> PPRPSSGELWGIHLMPPRILVECLLPNGMIVTLECLREATLITIKHELFKEARKYPLHQLLQDESSYIFVSVTQEAEREEFFDETRRLCDLRLFQPFLKVIEPVGNREEKILNREIGFAIGMPVCEFDMVKDPEVQDFRRNILNVCKEAVDLRDLNSPHSRAMYVYPPNVESSPELPKHIYNKLDKGQIIVVIWVIVSPNNDKQKYTLKINHDCVPEQVIAEAIRKKTRSMLLSSEQLKLCVLEYQGKYILKVCGCDEYFLEKYPLSQYKYIRSCIMLGRMPNLMLMAKESLYSQLPMDCFT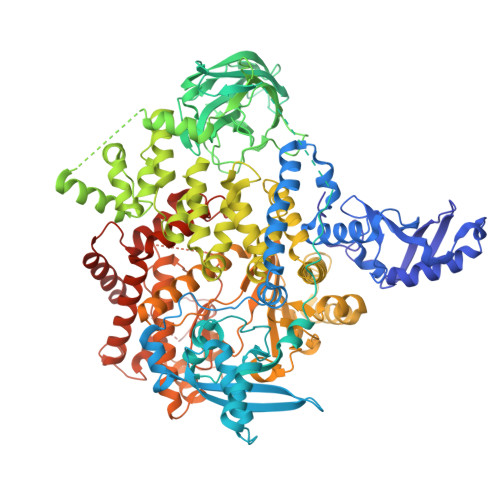MPSYSRRISTATPYMNGETSTKSLWVINSALRIKILCATYVNVNIRDIDKIYVRTGIYHGGEPLCDNVNTQRVPCSNPRWNEWLNYDIYIPDLPRAARLCLSICSVKGRKGAKEEHCPLAWGNINLFDYTDTLVSGKMALNLWPVPHGLEDLLNPIGVTGSNPNKETPCLELEFDWFSSVVKFPDMSVIEEHANWSVSREAGFSYSHAGLSNRLARDNELRENDKEQLKAISTRDPLSEITEQEKDFLWSHRHYCVTIPEILPKLLLSVKWNSRDEVAQMYCLVKDWPPIKPEQAMELLDCNYPDPMVRGFAVRCLEKYLTDDKLSQYLIQLVQVLKYEQYLDNLLVRFLLKKALTNQRIGHFFFWHLKSEMHNKTVSQRFGLLLESYCRACGMYLKHLNRQVEAMEKLINLTDILKQEKKDETQKVQMKFLVEQMRRPDFMDALQGFLSPLNPAHQLGNLRLEECRIMSSAKRPLWLNWENPDIMSELLFQNNEIIFKNGDDLRQDMLTLQIIRIMENIWQNQGLDLRMLPYGCLSIGDCVGLIEVVRNSHTIMQIQCKGGLKGALQFNSHTLHQWLKDKNKGEIYDAAIDLFTRSCAGYCVATFILGIGDRHNSNIMVKDDGQLFHIDFGHFLDHKKKKFGYKRERVPFVLTQDFLIVISKGAQECTKTREFERFQEMCYKAYLAIRQHANLFINLFSMMLGSGMPELQSFDDIAYIRKTLALDKTEQEALEYFMKQMNDAHHGGWTTKMDWIFHTIKQHALN(2,4,6-trimethylbenzene-1,3,5-triyl)trimethanol | C12 H18 O3 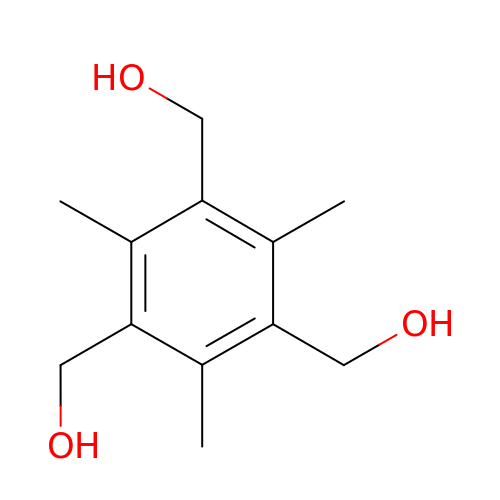| RZPWWYFQBDXLBQ-UHFFFAOYSA-N> MLEGKVKWFNSEKGFGFIEVEGQDDVFVHFSAIQGEGFKTLE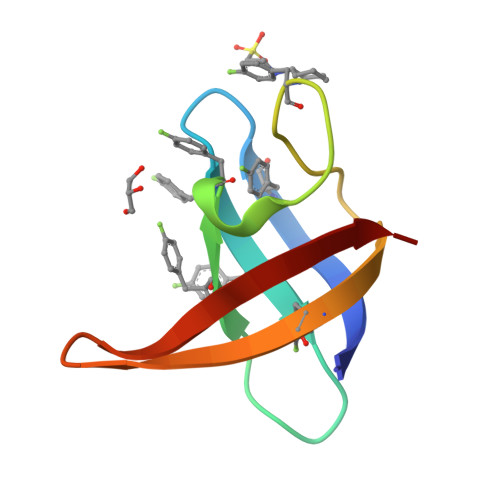EGQAVSFEIVEGNRGPQAANVTKE>[8x]GSHMKFPGKRKSKHYFPVNARDPLLQQFQPENETSAAWVVGIDQTLVDIEAKVDDEFIERYGLSAGHSLVIEDDVAEALYQELKQKNLITHQFAGGTIGNTMHNYSVLADDRSVLLGVMCSNIEIGSYAYRYLCNTSSRTDLNYLQGVDGPIGRCFTLIGESGERTFAISPG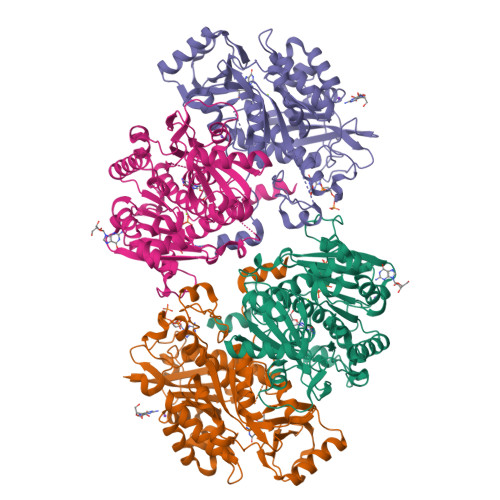HMNQLRAESIPEDVIAGASALVLTSYLVRCKPGEPMPEATMKAIEYAKKYNVPVVLTLGTKFVIAENPQWWQQFLKDHVSILAMNEDEAEALTGESDPLLASDKALDWVDLVLCTAGPIGLYMAGFTEDEAKRKTQHPLLPGAIAEFNQYEFSRAMRHKDCQNPLRVYSHIAPYMGGPEKIMNTNGAGDGALAALLHDITANSYHRSNVPNSSKHKFTWLTYSSLAQVCKYANRVSYQVLNQHSPRLTRGLPEREDSLEESYWDR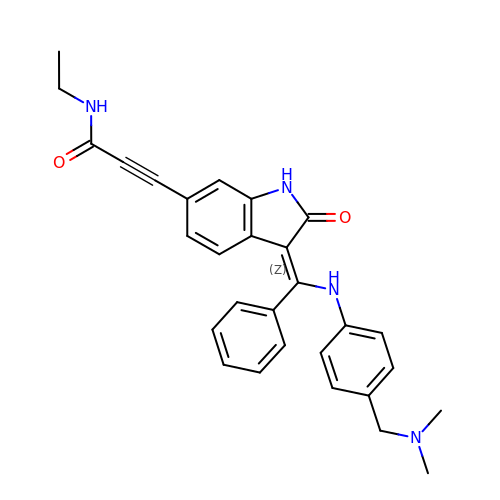3-[(3~{Z})-3-[[[4-[(dimethylamino)methyl]phenyl]amino]-phenyl-methylidene]-2-oxidanylidene-1~{H}-indol-6-yl]-~{N}-ethyl-prop-2-ynamide | C29 H28 N4 O2 | FLBNLJLONKAPLR-DQSJHHFOSA-N>GSVESHPVLEKLKAAHSYNPKEFEWNLKSGRVFIIKSYSEDDIHRSIKYSIWCSTEHGNKRLDSAFRCMSSKGPVYLLFSVNGSGHFCGVAEMKSPVDYGTSAGVWSQDKWKGKFDVQWIFVKDVPNNQLRHIRLENND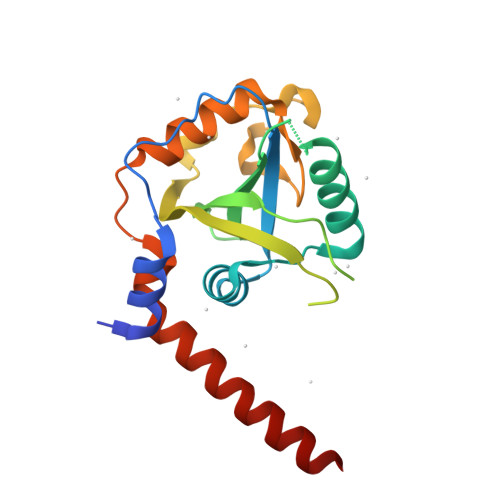NKPVTNSRDTQEVPLEKAKQVLKIISSYKHTTSIFDDFAHYEKRQEEEEVVRKERQSRNKQ[4x]> VPGPEYKVAILTVSDTVSAGAGPDRSGPRAVSVVDSSSEKLGGAKVVATAVVPDEVERIK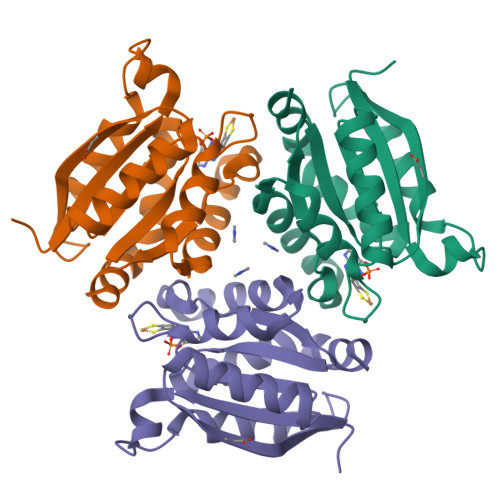DILQKWSDVDEMDLILTLGGTGFTPRDVTPEATKKVIERETPGLLFVMMQESLKITPFAMLSRSAAGIRGSTLIINMPGNPNAVAECMEALLPALKHALKQIA>[2x]TRDQNGTWEMESNENFEGYMKALDIDFATRKIAVRLTQTKVIDQDGDNFKTKTTSTFHHHHHHRNYDVDFTVGVEFDEYTKSLDNRHVKALVTWEGDVLVC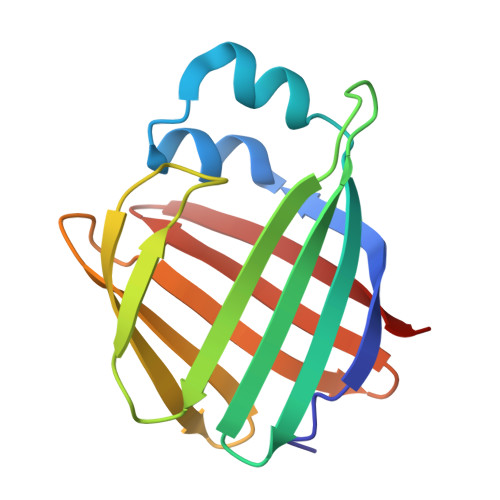VQKGEKENRGWKQWIEGDKLYLELTCGDQVCRQVFKKK> LSITTPEEMIEKAKGETAYLPCKFTLSPEDQGPL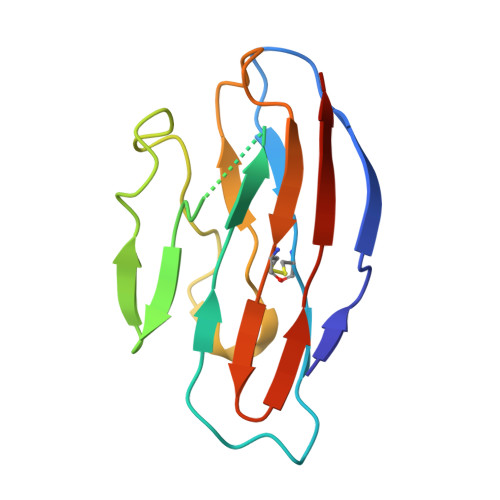DIEWLISPADNQKVDQVIILYSGDKIYDDYYPDLKGRVHFTSNDLKSGDASINVTNLQLSDIGTYQCKVKKAPGVANKKIHLVVLVK>[2x]MMSETAPLPSASSALEDKAASAPVVGIIMGSQSDWETMRHADALLTELEIPHETLIVSANRTPDRLADYARTAAERGLNVIIAGAGGAAHLPGMCAAWTRLPVLGV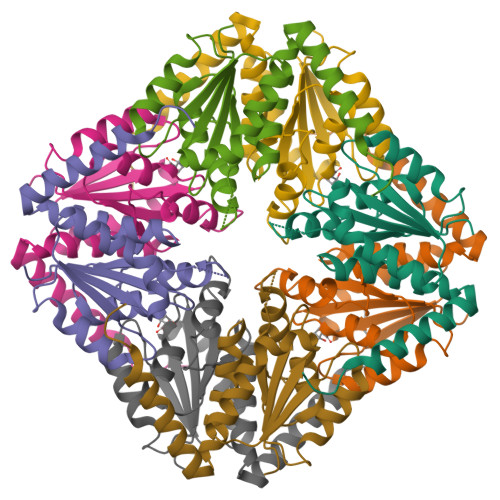PVESRALKGMDSLLSIVQMPGGVPVGTLAIGASGAKNAALLAASILALYNPALAARLETWRALQTASVPNSPITEDK> GSSLPKPILRVQPDSVVSRWTKVTFFCEETIGANEYRLYKDGKLYKTVTKNKQKPANKAEFSLSNVDLSNAGQYECSYSTQYKSSGYSDPLKLVVTGHYWTPSLLAQASPVVTSGGYVTLQCESWHNDHKFILTVEGPQKLSWTQDSQYNYSTRKYHALFSVGPVTPNQRWICRCYSYDRNRPYVWSPPSESVELLVSGNLQKPTIKAEPGSVITSKRAMTIWCQGNLDAEVYFLHNEGSQKTQSTQTLQQPGNKGKFFIPSMTRQHAGQYRCYCYGSAGWSQPSDTLELVVTGIYEHYKPRLSVLPSPVVTAGGNMTLHCASDFHYDKFILTKEDKKFGNSLDTEHISSSRQYRALFIIGPTTPTHTGTFRCYGYFKNAPQLWSVPSDLQQILISGLSKKPSLLTHQGHILDPGMTLTLQCYSDINYDRFALHKVGGADIMQHSSQQTDTGFSVANFTLGYVSSSTGGQYRCYGAHNLSSEWSASSEPLDILITGQLPLTPSLSVKPNHTVHSGETVSLLCWSMDSVDTFILSKEGSAQQPLRLKSKSHDQQSQAEFSMSAVTSHLSGTYRCYGAQNSSFYLLSSASAPVEL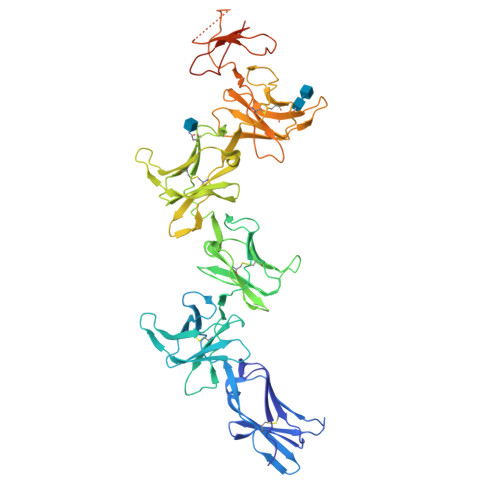TVSGAAAHHHHHH>APQQINDIVHRTITPLIEQQKIPGMAVAVIYQGKPYYFTWGYADIAKKQPVTQQTLFELGSVSKTFTGVLGGDAIARGEIKLSDPTTKYWPELTAKQWNGITLLHLATYTAGGLPLQVPDEVKSSSDLLRFYQNWQPAWAPGTQRLYANSSIGLFGALAVKPSGLSFEQAMQTRVFQPLKLNHTWINVPPAEEKNYAWGYREGKAVHVSPGALDAEAYGVKSTIEDMARWVQSNLKPLDINEKTLQQGIQLAQSRYWQTGDMYQGLGWEMLDWPVNPDSIINGSDNKIALAARPVKAITPPTPAVRASWVHKTGATGGFGSYVAFIPEKELGIVMLANKNYPNPARVDAAWQILNALQ[4x]

To enable future efforts on the optimization of bicyclic boronates, we report crystallographic and kinetic studies on inhibition of the clinically important class C AmpC β-lactamase from Escherichia coli (AmpCEC) by TAN, a previously reported model bicyclic boronate 2 (CB2), and a thioether bicyclic boronate derivative (CB3) that we have recently shown to have enhanced potency against some SBLs and MBLs in vitro. Many β-lactamases are encoded by plasmids, but the AmpC type β-lactamases that are present in most Escherichia coli strains are chromosomally encoded. While normally expressed at low levels, mutations in the ampC gene promoter and/or attenuator regions can lead to constitutive hyperproduction of AmpC in E. coli. In all three structures, analysis of the electron density maps for the AmpCEC active site indicates that the bicyclic boronates CB2, TAN, and CB3 have reacted with the nucleophilic S64 to form an anionic tetrahedral species in which the boron is sp3 hybridized, as observed for other bicyclic boronate SBL complex structures.

AmpCEC was co-crystallized with CB2 giving crystals with four molecules in each asymmetric unit, all of which manifested clear and continuous electron density for the covalently bound CB2 at the active site. The overall folds and orientations of active site residues and CB2 are very similar in all four chains (main chain RMSD of Chain B, C and D in relation to chain A: 0.31, 0.28, and 0.33 Å, respectively). Binding of the bicyclic boronate core of CB2, together with that of the amido side chain group portion, is very similar to that observed for TAN (CB3 has a different type of side chain). Interestingly, in the CB2 structure, the side chain of Q120 is directed away from the active site in all four molecules in the asymmetric unit; Q120 interacts with a water molecule (‘w’, observed in all chains of the ASU), which in turn interacts with the carbonyl oxygen of the acylamino CB2 side chain. Although the AmpCEC-CB2 complex was co-crystallized using a different crystallization condition than for the two other structures reported here, because the Q120 side chain does not interact with residues of other AmpCEC molecules in the crystalline lattice, reorientation due to formation of crystal contacts seems unlikely. In a crystal structure of AmpCEC, obtained by soaking with CB2, partial density for the bound CB2 was observed in the active site, though reorientation of the Q120 side chain was not observed (data not shown, because of poor electron density for the CB2 C-3 side chain). It is thus unclear whether the different orientation of Q120 compared to apo-AmpCEC is due to the different crystallization conditions or due to a specific feature of CB2 binding. The positioning of the Q120 side chain could impact on the potency of inhibition by bicyclic boronates containing an amido side chain, as in CB2 and TAN.>KDAIEEKFRERLKELVVPKHVMDVVDEELSKLGLLDNHSSEFNVTRNYLDWLTSIPWGKYSNENLDLARAQAVLEEDHYGMEDVKKRILEFIAVSQLRGSTQGKILCFYGPPGVGKTSIARSIARALNREYFRFSVGGMTDVAEIKGHRRTYVGAMPGKIIQCLKKTKTENPLILIDEVDKIGRGYQGDPSSALLELLDPEQNANFLDHYLDVPVDLSKVLFICTANVTDTIPEPLRDRMEMINVSGYVAQEKLAIAERYLVPQARALCGLDESKAKLSSDVLTLLIKQYCRESGVRNLQKQVEKVLRKSAYKIVSGEAESVEVTPENLQDFVGKPVFTVERMYDVTPPGVVMGLAWTAMGGSTLFVETSLRRPQDKDAKGDKDGSLEVTGQLGEVMKESARIAYTFARAFLMQHAPANDYLVTSHIHLHVPEGATPKDGPSAGCTIVTALLSLAMGRPVRQNLAMTGEVSLTGKILPVGGIKEKTIAAKRAGVTCIVLPAENKKDFYDLAAFITEGLEVHFVEHY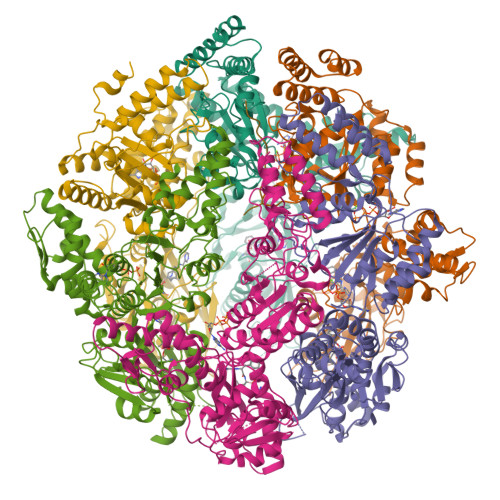REIFDIAF[6x]>PVPRSCAEPAGIPALLSPRDKLAQLLVVGVRDAADAQAVVTNYHVGGILIGSDTDLTIFDGALAEIVAGGGPLPLAVSVDEEGGRVSRLRSLIGGTGPSARELAQTRTVQQVRDLARDRGRQMRKLGITIDFAPVVDVTDAPDDTVIGDRSFGSDPATVTAYAGAYAQGLRDAGVLPVLKHFPGHGRGSGDSHNGGVTTPPLDDLVGDDLVPYRTLVTQAPVGVMVGHLQVPGLTGSEPASLSKAAVNLLRTGTGYGAPPFDGPVFSDDLSGMAAISDRFGVSEAVLRTLQAGADIALWVTTKEVPAVLDRLEQALRAGELPMSAVDRSVVRVATMKGPNPGC[2x]

Despite the absence of other known PG-recycling proteins, we have shown that LpqI is an authentic exo-acting β-N-acetylglucosaminidase, which is able to cleave PG fragments in vitro. In previously characterised PG-recycling systems free amino sugars are produced by NagZ, which belongs to the CAZy glycoside hydrolase family 3 (GH3). The β-N-acetylglucosaminidase sub-family including all known NagZ enzymes utilise a conserved Asp-His catalytic dyad, which has been well characterised. As a lipoprotein LpqI is expected to be found attached to the external face of the cytoplasmic membrane, which is consistent with proteomics results.

To test this, we cloned, expressed and purified LpqITB using an N-terminal His6-SUMO tag, which was subsequently cleaved from the protein. LpqI consists of a single TIM-barrel domain similar to cytoplasmic Gram-negative orthologs but lacks the C-terminal domain associated with extracellular NagZ enzymes from some Gram-positive bacteria. Superposition of the post-cleavage NagZPa complex with LpqI indicates that the appropriate coordinating residues for MurNAc or 1,6-anhydroMurNAc recognition are intact in LpqI, supporting its role in PG-recycling. The only detectable activity for LpqI was with GlcNAc-containing substrates. The Michaelis–Menten constants (kcat = 2.0 × 10–2 ± 0.04 × 10–2 s−1 and Km = 72 ± 5 µm) of LpqI using 4MU-GlcNAc as a substrate were found to be similar to other NagZ enzymes using this substrate. In a similar assay we were also able to show that LpqI releases GlcNAc from soluble PG fragments, including PG fragments with a 1,6-anhdroMurNAc terminus. In this assay, LpqI was not observed to release any soluble PG in contrast to the muramidase mutanolysin. Together these data support the role of LpqI as an exo-acting enzyme involved in fragment recycling, rather than as an endo-acting autolysin. From these experiments, we concluded that LpqI is involved in amino sugar recovery but is not required for stem-peptide recycling. In contrast to inhibition of P. aeruginosa NagZ, deletion of lpqI resulted in an increase in survival in the presence of lysozyme and all cell wall active antibiotics tested.> 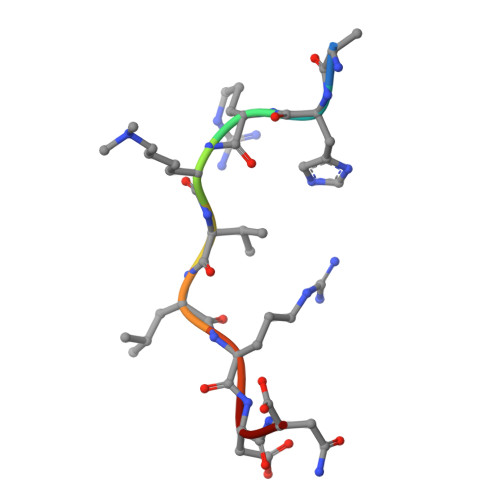RHRKVLRDN>AMSYTPGQPVTAVVQRVEIHKLRQGENLILGFSIGGGIDQDPSQNPFSEDKTDKGIYVTRVSEGGPAEIAGLQIGDKIMQVNGWDMTMVTHDQARKRLTKRSEEVVRLLVTRQ[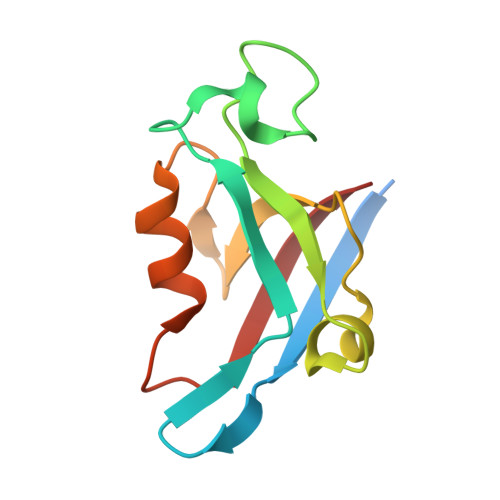4x]>[2x]MRVLVSNDDGVDAPGIKILADALRNAGHEVMVVAPDRDRSGASNSLTLDTPIRAKQIDMHTYSVAGTPTDCVHLALTGLLNYDPDIVVSGINNTGNLGDDVIYSGTVSAAMEGRFLGLPAVAVSLVTLYREGQQAPQYETAAHAAINI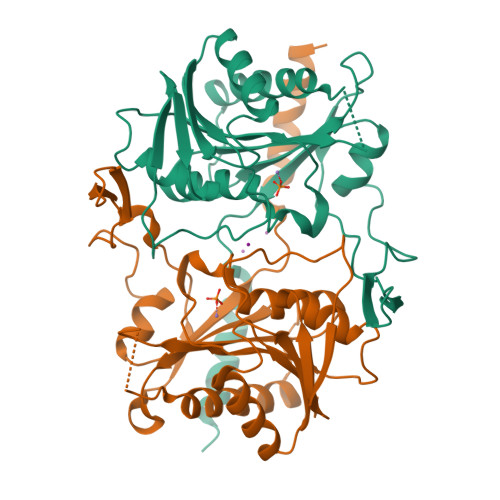VAQLKTDPLPADTILNVNVPDVTWQQMRGFKVTRLGNRHRSAPCLTQTDPRGHTIYWIGPAGPEQDAGPGTDFDAVRNTYISITPIHVDLTRYQALENVTRWTDRLTAHMDWPTLEHHHHHH> MQVNRLPFFTNHFFDTYLLISEDTPVGSSVTQLLARDMDNDPLVFGVSGEEASRFFAVEPDTGVVWLRQPLDRETKSEFTVEFSVSDHQGVITRKVNIQVGDVNDNAPTFHNQPYSVRIPENTPVGTPIFIVNATDPDLGAGGSVL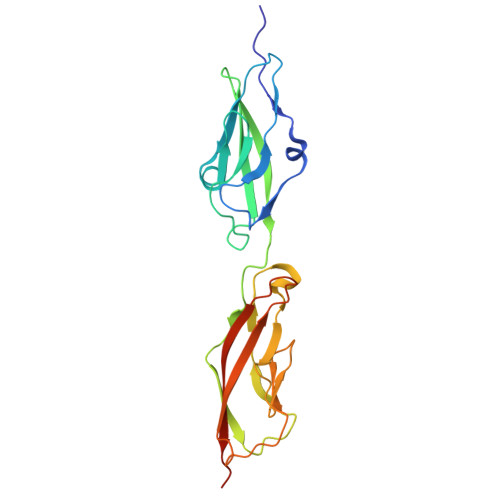YSFQPPSPFFAIDSARGIVTVIQELDYEVTQAYQLTVNATDQDKTRPLSTLANLAIIITDLEHHHHHH(3R,5R)-3,5-dihydroxy-7-[(1S,2S,8S,8aR)-2-methyl-8-{[(2S)-2-methylbutanoyl]oxy}-1,2,6,7,8,8a-hexahydronaphthalen-1-yl]heptanoic acid | C23 H36 O6 | 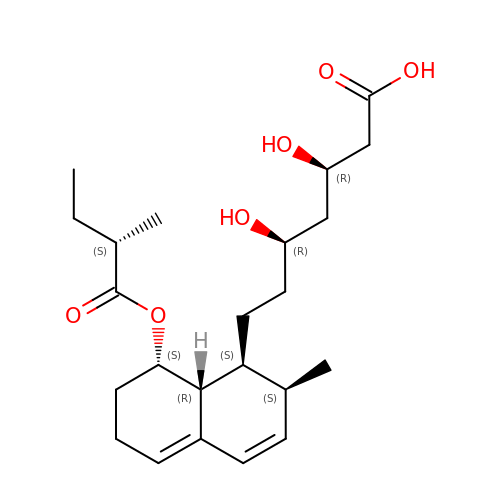BOZILQFLQYBIIY-INTXDZFKSA-N>HEDEIKKLRTSGSMTQNPHEVARVRNLNRIIMGKYEIEPWYFSPYPIELTDEDFIYIDDFTLQYFGSKKQYERYRKKCTLRHPPGNEIYRDDYVSFFEIDGRKQRTWCRNLCLLSKLFLDHKTLYYDVDPFLFYCMTRRDELGHHLVGYFSKEKESADGYNVACILTLPQYQRMGYGKLLIEFSYELSKKENKVGSPEKPLSDLGLLSYRAYWSDTLITLLVEHQKEITIDEISSMTSMTTTDILHTAKTLNILRYYKGQHIIFLNEDILDRYNRLKAKKRRTIDPNRLIWKPPVFTASQLRFAW[3x];>MTDELKSYEALKAELKKSLQDRREQEDTFDNLQQEIYDK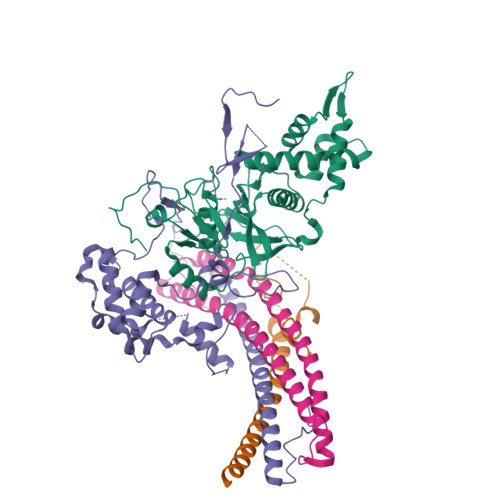ETEYFSHNSNNNHSGHGGAHGSKSHYSGNIIKGFDTFSKSHHSHADSAFNNNDRIFSLSSATYVKQQHGQSQND[3x];>SSNSRFRHRKISVKQHLKIYLPNDLKHLDKDELQQREVVEIETGVEKNEEKEVHLHRILQMGSGHTKHKDYIPTPDASMTWNEYDKFYTGSFQETTSYIKFSATVEDCCGTNYNMDERDETFLNEQVNKGSSDILTEDEFEILCSSFEHAIHERQPFLSMDPESILSFEELKPTLIKSDMADFNLRNQLNHEINSHKTHFITQFDPVSQMNTRPLIQLIEKFGSKIYDYWRERKIEVNGYEIFPQLKFERPGEKEEIDPYVCFRRREVRHPRKTRRIDILNSQRLRALHQELKNAKDLALLVAKRENVSLNWINDELKIFDQRVKIKNLKRSLNISGEDDDLINHKRKRPT[3x];>MDPSLVLEQTIQDVSNLPSEFRYLLEEIGSNDLKLIEEKKKYEQKESQIHKFIRQQGSIPKHPQEDGLDKEIKESLLKCQSLQREKCVLANTALFLIARHLNKLEKNIALLEEDGVLAPV[3x]> MGSSHHHHHHSSGRENLYFQGHMNGDQNSDVYAQEKQDFVQHFSQIVRVLTEDEMGHPEIGDAIARLKEVLEYNAIGGKYNRGLTVVVAFRELVEPRKQDADSLQRAWTVGWCVELLQAFFLVADDIMDSSLTRRGQICWYQKPGVGLDAINDANLLEACIYRLLKLYCREQPYYLNLIELFLQSSYQTEIGQTLDLLTAPQGNVDLVRFTEKRYKSIVKYLTAFYSFYLPIAAAMYMAGIDGEKEHANAKKILLEMGEFFQIQDDYLDLFGDPSVTGKIGTDIQDNK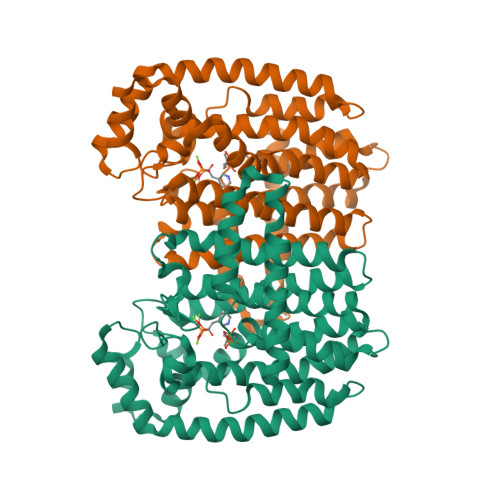CSWLVVQCLQRATPEQYQILKENYGQKEAEKVARVKALYEELDLPAVFLQYEEDSYSHIMALIEQYAAPLPPAVFLGLARKIYKRRK>[2x]MT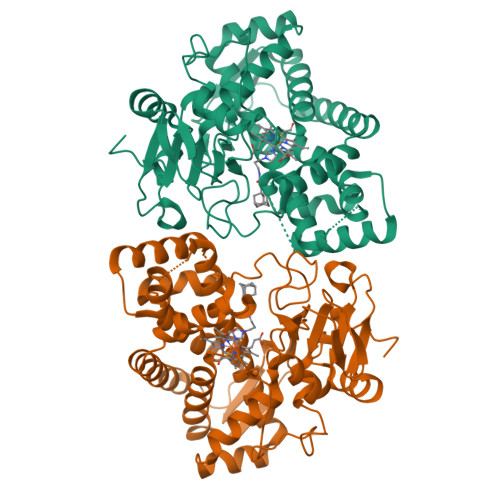TAAGLSGIDLTDLDNFADGFPHHLFAIHRREAPVYWHRPTEHTPDGEGFWSVATYAETLEVLRDPVTYSSVTGGQRRFGGTVLQDLPVAGQVLNMMDDPRHTRIRRLVSSGLTPRMIRRVEDDLRRRARGLLDGVEPGAPFDFVVEIAAELPMQMICILLGVPETDRHWLFEAVEPGFDFRGSRRATMPRLNVEDAGSRLYTYALELIAGKRAEPADDMLSVVANATIDDPDAPALSDAELYLFFHLLFSAGAETTRNSIAGGLLALAENPDQLQTLRSDFELLPTAIEEIVRWTSPSPSKRRTASRAVSLGGQPIEAGQKVVVWEGSANRDPSVFDRADEFDITRKPNPHLGFGQGVHYCLGANLARLELRVLFEELLSRFGSVRVVEPAEWTRSNRHTGIRHLVVELRGG> KVSEQLKCCSGILKEMFA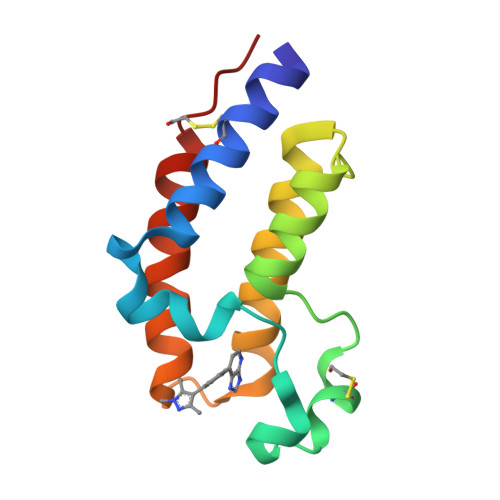KKHAAYAWPFYKPVDVEALGLHDYCDIIKHPMDMSTIKSKLEAREYRDAQEFGADVRLMFSNCYKYNPPDHEVVAMARKLQDVFEMRFAKMPDE> GQVKFFTDVNSKQIKTLQVKVAGELISEPYIALGGEEQIEINFDGLGSGYTRYAYNVVHCNADWTQSQLSPIEYMNGFQGTTIDDFANSIGTTTQYSNYRLLLPNDDVQFKVSGNYAIQVYNEDTPDQIIFTACFSVVEPVVNISASVSGNTDIDTNQSHQQVSFNINNKNFPITYPQT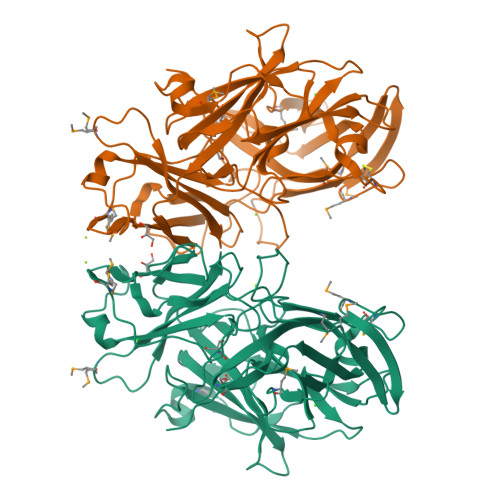DLKIFVYQDNRRDNAVTDLQPMSILENQISYTYNRNLIFPAGNEYRRMEFLSNKYNGMHVENISFHNPYYNVELMTDYRRDKGTYQYDQDQDGRFFIRCSDCNDPDTEADYYIVHFTLACDPLPDGSVYLNGELFNNVLDEKSKMGYNFETKQYEKAVLLKQGSYNYQYLFVPTGSSVGQTGPIEGNYYQTQNEYSIYVYYRPMGARYDRLIGVTTVRNEMQVF>[2x]HHHHHHAEKASLQLNQQQKELVQILLGAHTRHVGPLFDQFVQFKPPAYLFMHHRPFQPRGPVLPLLTHFADINTFMVQQIIKFTKDLPLFRSLTMEDQISLLKGAAVEILHISLNTTFCLQTENFFCGPLCYKMEDAVHAGFQYEFLESILHFHKNLKGLHLQEPEYVLMAATALFSPDRPGVTQREEIDQLQEEMALILNNHI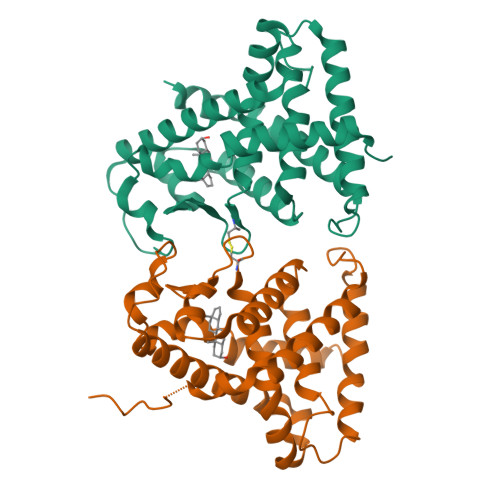MEQQSRLQSRFLYAKLMGLLADLRSINNAYSYELQRLEELSAMTPLLGEICS> MLAHEIRARVARGEVSPLEVAQAYLKRVQELDPGLGAFLSLNERLLEEAEAVDPGLPLAGLVVAVKDNIATRGLRTTAGSRLLENFVPPYEATAVARLKALGALVLGKTNLDEFGMGSSTEHSAFFPTKNPFDPDRVPGGSSGGSAAALAADLAPLALGSDTGGSVRQPAAFCGVYGLKPTYGRVSRFGLIAYASSL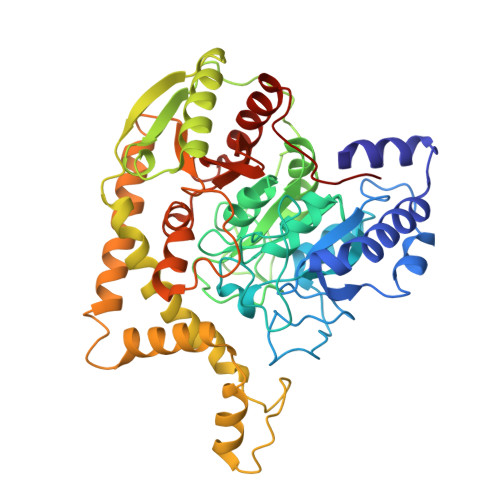DQIGPMARSVRDLALLMDAAAGPDPLDATSLDLPPRFQEALEGPLPPLRLGVVREALAGNSPGVERALEEALKVFRELGLSVREVSWPSLPQALAAYYILAPAEASSNLARYDGTLYGRRAAGEEVEGMMEATRALFGLEVKRRVLVGTFVLSSGYYEAYYGRAQAFRRRLKAEAQALFREVDLLLLPTTPHPAFPFGARRDPLAMYREDLYTVGANLTGLPALSFPAGFEGHLPVGLQLLAPWGEDERLLRAALAFEEATARAHLKAPLGEAL(3E)-3-iminooxepin-2(3H)-one | C6 H5 N O2 | 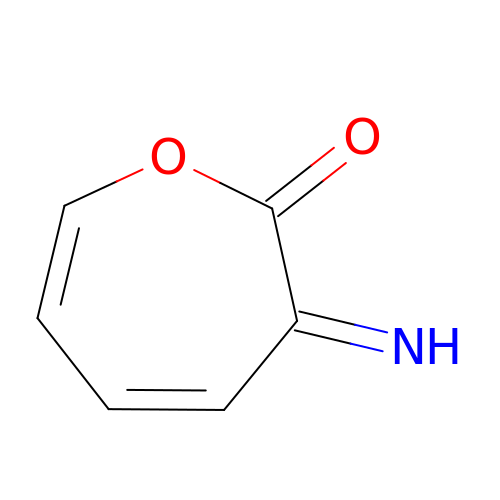HQPIXVSGYRVKOL-FNORWQNLSA-N>[4x]MEEDKLALGREIFLERSEPQCALCHTLADAEAVGEVGPNLDELKPDAERVNTAVTNGIGPMPANEILTDEEIEAVALYVSTVAGKAKNSSSVDKLAAALEHHHHHH

In most cells, the detoxification of sulfite by oxidation to sulfate (Equation 1) is catalyzed by sulfite oxidizing enzymes (SOEs). Here, we have investigated an electron transfer complex involving the periplasmic SorT sulfite dehydrogenase from the α-Proteobacterium Sinorhizobium meliloti, which represents a structurally uncharacterized type of SOE, and its electron acceptor, the c-type cytochrome SorU. In S. meliloti the SorT sulfite dehydrogenase is part of a sulfite detoxification system that is induced in response to the degradation of sulfur containing substrates such as the organosulfonate taurine. Electrons derived from sulfite oxidation are passed on to the SorU cytochrome, and likely then to cytochrome oxidase, as S. meliloti is capable of sulfite respiration.

The structure of the SorU protein, both within the SorT/SorU complex and when crystallized in isolation, is predominantly α-helical with three major α-helices arranged to form a bundle that frames the heme-binding site (C47XXC50H, axial ligands: His 51 and Met 87). Unlike other known cytochromes c that can act as electron acceptors to SOEs, the electrostatic surface of SorU has an overall negative charge. A surface loop on SorU (residues 82–93) moves away from the SorT/SorU complex interface, leading to a reorientation of the heme ligand residue Met 87 so that a different Met 87 rotamer coordinates the iron in the SorU structures within and outside of the complex. Changes in the conformation of axial heme ligands are known to alter the orbital interactions between the iron atom and the ligand, which can change the redox properties of the heme group. Small (ca. 20 × 10 × 10 μ) crystals of SorU were grown in drops containing equal volumes (2 μL) of protein and reservoir solution (1.8 M tri-sodium citrate, pH 5.5, 0.1 M glycine), which were harvested and flash-cooled in liquid nitrogen without additional cryoprotection. The refined SorU model, from the SorT/SorU complex structure, was used as a search model to solve the SorU structure by molecular replacement using PHASER. Refinement was carried out with REFMAC5 and PHENIX and converged with residuals R= 0.192 and Rfree = 0.240.methyl 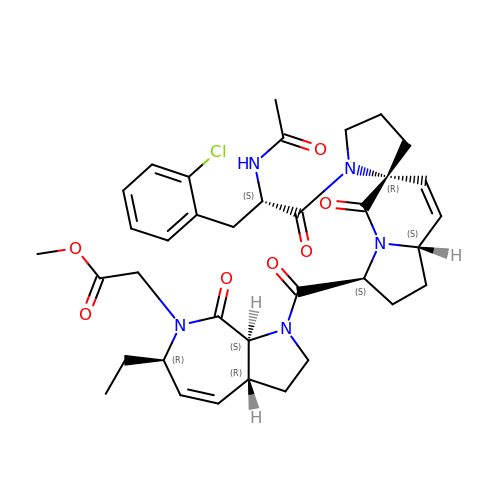2-[(3~{a}~{R},6~{R},8~{a}~{S})-1-[(3~{S},6~{R},8~{a}~{S})-1'-[(2~{S})-2-acetamido-3-(2-chlorophenyl)propanoyl]-5-oxidanylidene-spiro[1,2,3,8~{a}-tetrahydroindolizine-6,2'-pyrrolidine]-3-yl]carbonyl-6-ethyl-8-oxidanylidene-3,3~{a},6,8~{a}-tetrahydro-2~{H}-pyrrolo[2,3-c]azepin-7-yl]ethanoate | C36 H44 Cl N5 O7 | VSCCVWMHHYBOGJ-WZYZTGQKSA-N> GPLGSMKDILSNYSNLIYLNKYVKEKDKYINDYRIIRTLNQGKFNKIILCEKDNKFYALKKYEKSLLEKKRDFTKSNNDKISIKSKYDDFKNELQIITDIKNEYCLTCEGIITNYDEVYIIYEYMENDSILKFDEYFFVLDKNYTCFIPIQVIKCIIKSVLNSFSYIHNEKNICHRDV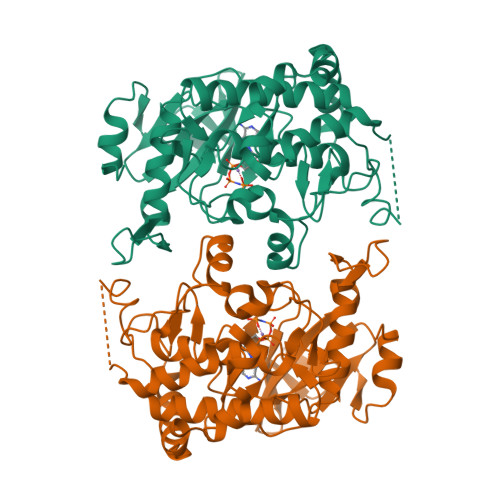KPSNILMDKNGRVKLSDFGESEYMVDKKIKGSRGTYEFMPPEFFSNESSYNGAKVDIWSLGICLYVMFYNVVPFSLKISLVELFNNIRTKNIEYPLDRNHFLYPLTNKKSTCSNNFLSNEDIDFLKLFLRKNPAERITSEDALKHEWLADTNIEDLREFSKELYKKRKKL>[4x]MSLDFNTLAQNFTQFYYNQFDTDRSQLGNLYRNESMLTFETSQLQGAKDIVEKLVSL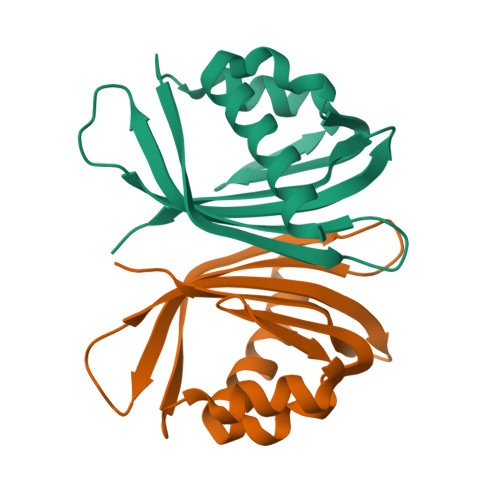PFQKVQHRITTLDAQPASPYGDVLVMITGDLLIDEEQNPQRFSQVFHLIPDGNSYYVFNDIFRLNYSA> KSTNSVSISGSTSVGPVMEAEAEAFKTKKPDVSIEINQIGSSAGIKNAMEGVS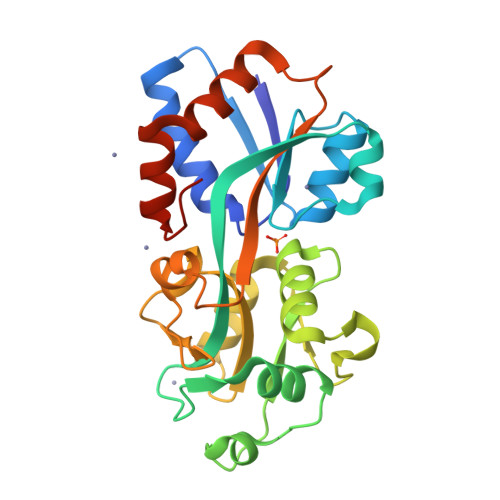EIGMASRDLKGEEKQAGLKEVEIAYDGIALITHKNNPVKDLTLVQIKDIYTGKITNWKELGGNDAPIVVVSREDGSGTRDAFQEIVGFKAEELTVNSQISDGSGNIKSLVQGNENAIGYISFSYVDDSVSAVKVDGVEATPENVLNKSYKVSRPFLAVYKEENLTESGKSFIDFILSEEGQDIVAKEHLIKVKHHHHHH>GPLGSDEGVVKEIPITHHVKEGYEKADPAQFELLKVLGQGSFGKVFLVRKKTGPDAGQLYAMKVLKKASLKVRDRVRTKMERDILVEVNHPFIVKLHYAFQTEGKLYLILDFLRGGDVFTRLSKEVLFTEEDVKFYLAELALALDHLHQLGIVYRDLKPENILLDEIGHIKLTDFGLSKESVDQEKKAYSFCGTVEYMAPEVVNRRGHSQSADWWSYGVLMFEMLTGTLPFQGKDRNETMNMILKAKLGMPQFLSAEAQSLLRMLFKRNPANRLGSEGVEEIKRHLFFANI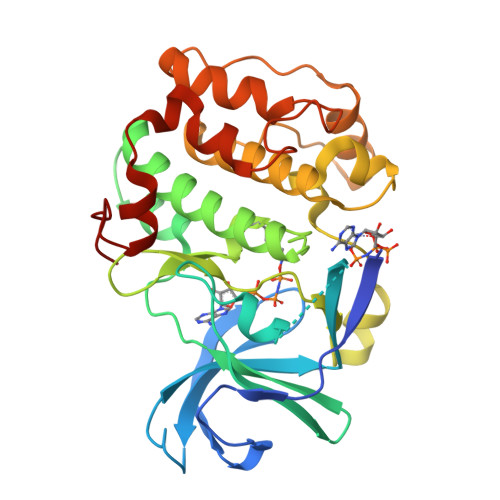DWDKLYKREVQPPFKP[2x]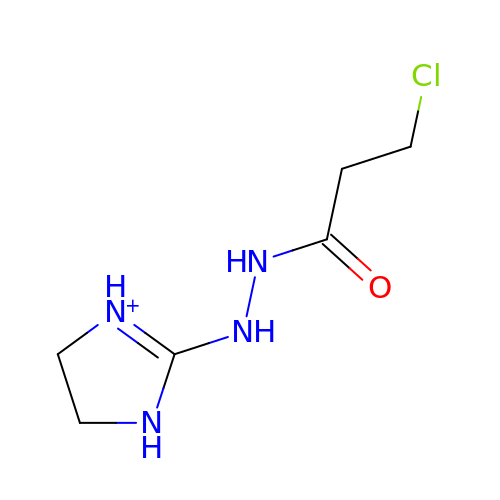3-chloranyl-~{N}'-(4,5-dihydro-1~{H}-imidazol-3-ium-2-yl)propanehydrazide | C6 H12 Cl N4 O | KIPZHINDKFZDKZ-UHFFFAOYSA-O>GGMILLIDNYDSFTWNLYQYFCELGADVLVKRNDALTLADIDALKPQKIVISPGPCTPDEAGISLDVIRHYAGRLPILGVCLGHQAMAQAFGGKVVRAAKVMHGKTSPITHNGEGVFRGLANPLTVTRYHSLVVEPDSLPACFDVTAWSETREIMGIRHRQWDLEGVQFHPESILSEQGHQLLANFLHR[2x];>GHMKTLSPAVITLLWRQDAAEFYFSRLSHLPWAMLLHSGYADHPYSRFDIVVAEPICTLTTFGKETVVSESEKRTTTTDDPLQVLQQVLDRADIRPTHNEDLPFQGGALGLFGYDLGRRFESLPEIAEQDIVLPDMAVGIYDWALIVDHQRHTVSLLSHNDVNARRAWLESQQFSPQEDFTLTSDWQSNMTREQYGEKFRQVQEYLHSGDCYQVNLAQRFHATYSGDEWQAFLQLNQANRAPFSAFLRLEQGAILSLSPERFILCDNSEIQTRPIKGTLPRLPDPQEDSKQAVKLANSAKDRAENLMIVDLMRNDIGRVAVAGSVKVPELFVVEPFPAVHHLVSTITAQLPEQLHASDLLRAAFPGGSITGAPKVRAMEIIDELEPQRRNAWCGSIGYLSFCGNMDTSITIRTLTAINGQIFCSAGGGIVADSQEEAEYQETFDKVNRILKQLEK[2x]

Here, we chose aminodeoxychorismate synthase (ADCS) from Escherichia coli, which consists of a class I glutaminase subunit (PabA) and a synthase subunit (PabB), to investigate the mechanism of glutaminase catalysis regulation and its impact on overall GAT activity. PabB catalyzes the amination of chorismate (Cho) to 4-amino-4-deoxy-chorismate, which is a committed step in folic acid biosynthesis. GATs comprise minimally a glutaminase that produces ammonia, which reacts with a synthase-bound substrate to yield specific nitrogen-containing products. As evidenced by analytical gel filtration and isothermal titration calorimetry (ITC) data, the PabA and PabB subunits form a heterodimeric assembly with a dissociation constant KD = 0.16 ± 0.06 μM.

When Gln was added to the crystallization buffer, we found a glutamyl thioester (Gln-TE) adduct covalently bound to the catalytic aC79 within the glutaminase active site in only one of the two PabA/PabB heterodimers, indicating that under the given crystallization conditions the glutaminase reaction proceeded only to the Gln-TE adduct without performing the final hydrolysis step. When Cho was subsequently added to these crystals, it was bound to the synthase active site of both ADCS heterodimers. Consistent with previous observations for related MST enzymes, the benzoate moiety of Cho is complexed by a magnesium ion. The central part of the tunnel is mainly formed by hydrophobic PabB residues and terminates next to the 4-hydroxy-1,5-cyclohexadiene-1-carboxylic acid ring of Cho, which is the reactive group for Cho transamination. In contrast, upon additional Cho and Mg2+ binding to the ADCS synthase active site, there were no further significant alterations in the PabA/PabB arrangement, consistent with only a minor regulatory effect of Cho/Mg2+ on glutaminase activity. In the ADCS structures with Gln-TE bound in the glutaminase active site, we consistently observed a distinct water molecule interacting with active site residues aY127 and aH168. This water molecule is in an appropriate position to hydrolyze the Gln-TE, as illustrated by a close distance of less than 3 Å to the Gln-TE reactive carbon atom, which is subject for nucleophilic acyl substitution, and hence it is referred to as the glutaminase catalytic water molecule. We also found several interactions between the noncatalytic amino group of Gln-TE and residues of both ADCS subunits, including bG207 and bY210 from the PabB subunit, allowing the catalytic center of Gln-TE to be positioned with very high spatial precision, to generate a catalytically competent glutaminase active site arrangement at the PabA/PabB interface. In this arrangement, the entire exposed Gln-TE surface not interacting with PabA residues (25 Å2) is buried by interactions with residues of the PabB subunit, demonstrating that the ADCS glutaminase active site is shared with the synthase subunit PabB.{(3R,5R,6S)-5-(3-chlorophenyl)-6-(4-chlorophenyl)-1-[(2S,3S)-2-hydroxypentan-3-yl]-3-methyl-2-oxopiperidin-3-yl}acetic 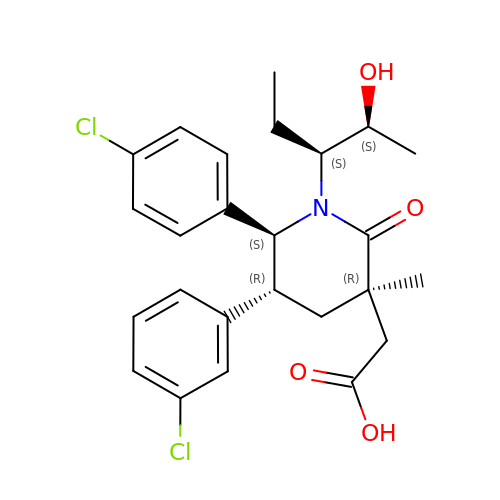acid | C25 H29 Cl2 N O4 | YUALYRLIFVPOHL-VPLUBSIMSA-N> GFQQSHYFVALYRFKALEKDDLDFRPGEKITVIDDSNEEWWRGKIGEKVGFFPPNF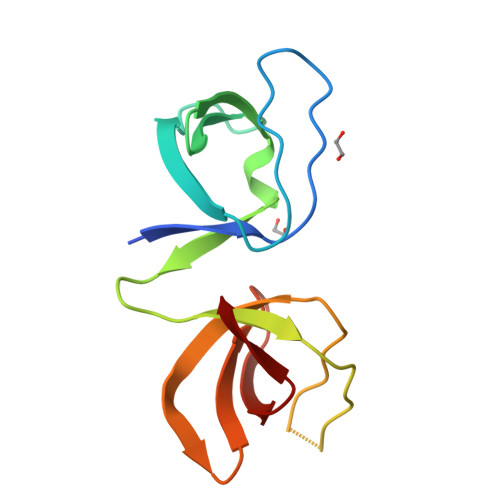IIRVRAGERVHRVTRSFVGNREIGQITLKKDQIVVQKGDEAGGYVKVYTGRKVGLFPTDFLEEI>MATTTVGLTDLKVRLVRDDFADAVAWVARSLPSRPTVPVLAGVLLTGSDDGLTISSFDYEVSAEVQIPAEIAAPGTVLVSGRLLSEITRALPNKPVDLSVEGTRVSLTCGSARFSLPTMAVEDYPALPELPAETGSVPADLFAEAIGQVAVAAGRDDTLPMLTGIRVEISGDRMVLAATDRFRLAVRELTWTTKTPDVEAAVLVPAKTLAEAAKTGLDGSEVQLALGAGPSVGQDGLLGIRSEGKRSTTRLLDAEFPKFRQLLPTEHTAMATIGVGELTEAIKRVALVADRGAQVRMEFADDVLHLSAGADDVGRA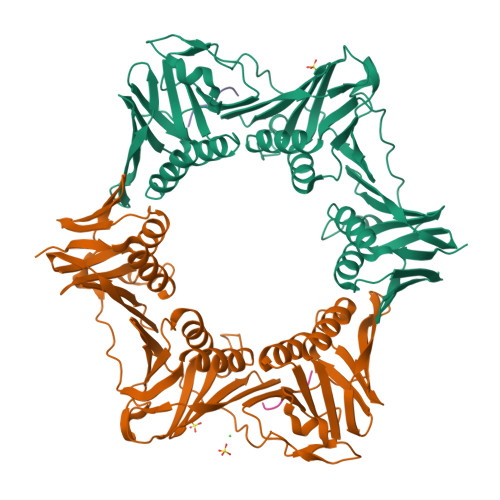EEDLPVSFSGEPLTIAFNPGYLTDGLGALHSERVTFGFTTPSKPAVLRPATEADAALNGNGPFPAAETDYVYLLMPVRLPG[4x];>[4x]QESLFA> MSGSLREEIRKLAEQLSEKYKDEEIRELAREAAELAEESDDPEVLELAYEALKKGLELEDEEKVKLILLAAVLAARVARGEVPEEKLEIALKALELAEASEDERIIRGALRAALAAARTDDPLALEVVLEALERAQASEDERLIRAILAAAYAFALLAVAGASAERLKEAEAIVKELIAAAEKGASPQELVLLVIEMMVKGMGVTMETHRSGNEVKVVIKGLHESQQEVLLEAVLFAAELMGVRVRIRFKGDTVTIVVREGSGSHHWGSTHHHHHH

Several natural systems exhibit ‘facilitated dissociation’, in which an effector (E) can bind to a target–host (TH) complex to form an excited ternary complex (THE)20–26 from which the target dissociates quickly. We set out to design protein systems that undergo facilitated dissociation. We use a switchable target binder (host) and a flexible effector that can rapidly bind to and switch the target–host complex to induce a large steric clash with the target, forming a strained excited ternary complex. We show here that by explicitly considering excited intermediate states when designing coupled protein systems, a broad range of facilitated dissociation systems can be designed.

We used X-ray crystallography to structurally characterize multiple states of our designed systems. For both the AS1 and the AS5 systems, the crystal structures of the hosts alone and of the host–effector complexes closely match the design models (maximum 1.3 Å Cα root mean square deviation (RMSD)). The unbound structures show an open hydrophobic cleft in the new designed state X poised to bind the effector, and the effector-bound structures show that binding the effector causes the two switch domains to register-shift into the designed state Y. Starting from AS0, we constructed a new state X by shifting the two domains from their state Y positions relative to each other (by one heptad along the helix of domain 1 that contacts domain 2), building a new loop between the domains, and optimizing single sequences that could adopt both this new state X and the original effector-bound state Y. This approach maintains the open cleft in state X by introducing minimal rotation from state Y and simplifies the multi-state sequence-design challenge by minimizing the local structural differences between the two states. Transition between conformational states occurs by a register shift throughout which the cleft could remain open and bind the effector.(2S,6S)-2-amino-6-[({3-hydroxy-2-methyl-5-[(phosphonooxy)methyl]pyridin-4-yl}methyl)amino]heptanedioic 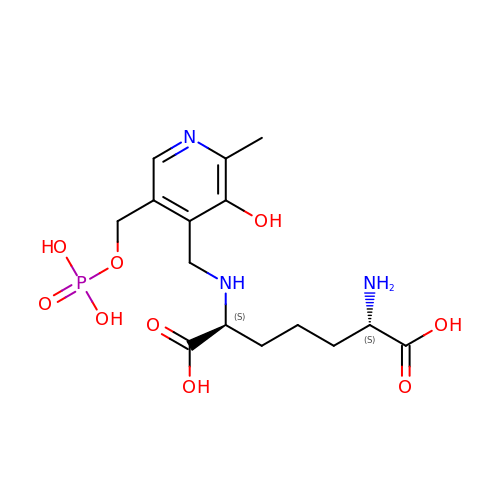acid | C15 H24 N3 O9 P | AEPLLCAFHXWECU-RYUDHWBXSA-N> GPLGSRRRVRAILPYTKVPDTDEISFLKGDMFIVHNELEDGWMWVT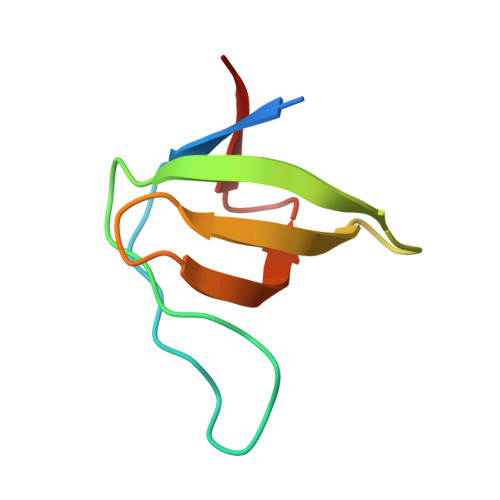NLRTDEQGLIVEDLVEEVGR>[6x]MHYLPVAIVTGATRGIGKAICQKLFQKGLSCIILGSTKESIERTAIDRGQLQSGLSYQRQCAIAIDFKKWPHWLDYESYDGIEYFKDRPPLKQKYSTLFDPCNKWSNNERRYYVNLLINCAGLTQESLSVRTTASQIQDIMNVNFMSPVTMTNICIKYMMKSQRRWPELSGQSARPTIVNISSILHSGKMKVPGTSVYSASKAALSRFTEVLAAEMEPRNIRCFTISPG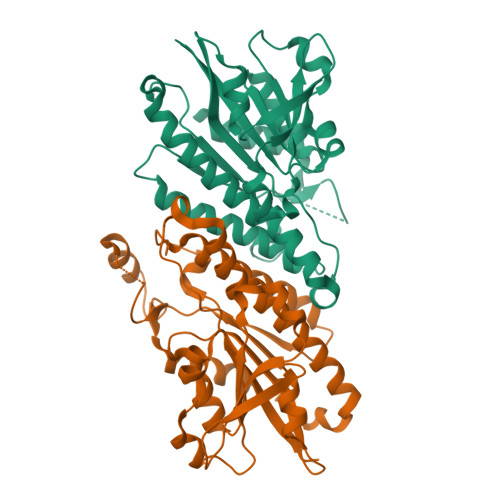LVKGTDMIQNLPVEAKEMLERTIGASGTSAPAEIAEEVWSLYSRTALETLEHHHHHH>AKIDNAVLPEGSLVLVTGANGFVASHVVEQLLEHGYKVRGTARSASKLANLQKRWDAKYPGRFETAVVEDMLKQGAYDEVIKGAAGVAHIASVVSFSNKYDEVVTPAIGGTLNALRAAAATPSVKRFVLTSSTVSALIPKPNVEGIYLDEKSWNLESIDKAKTLPESDPQKSLWVYAASKTEAELAAWKFMDENKPHFTLNAVLPNYTIGTIFDPETQSGSTSGWMMSLFNGEVSPALALMPPQYYVSAVDIGLLHLGCLVLPQIERRRVYGTAGTFDWNTVLATFRKLYPSKTFPADFPDQGQDLSK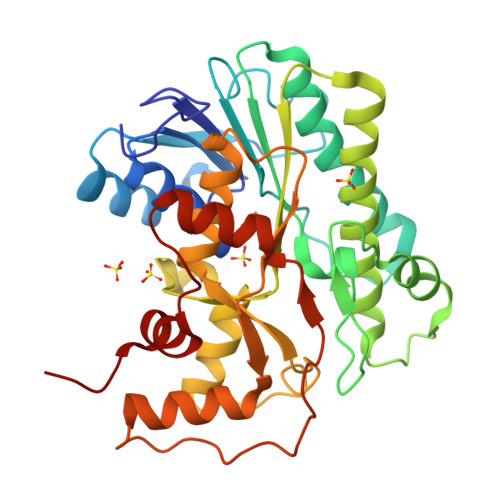FDTAPSLEILKSLGRPGWRSIEESIKDLVGSETA[2x]>GSHMPSELTPEERSELKNSIAEFHTYQLDPGSCSSLHAQRIHAPPELVWSIVRRFDKPQTYKHFIKSCSVEQNFEMRVGCTRDVIVISGLSANTSTERLDILDDERRVTGFSIIGGEHRLTNYKSVTTVHRFEKENRIWTVVLESYVVDMPEGNSEDDTRMFADTVVKLNLQKLATVAEAMARNSG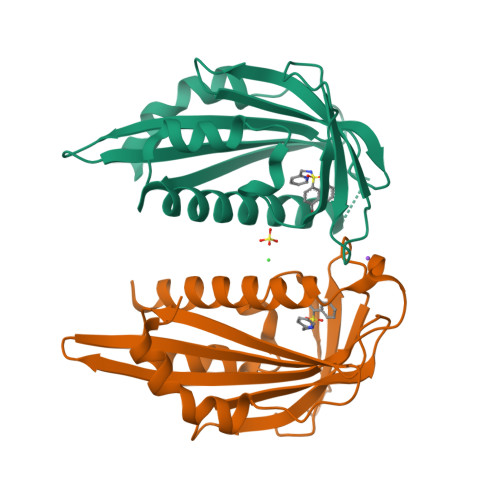DGSGSQVT[3x]>[12x]ETLVRPKPLLLKLLKSVGAQKDTYTMKEVLFYLGQYIMTKRLYDEKQQHIVYCSNDLLGDLFGVPSFSVKEHRKIYTMIYRNLVV;>[12x]XTSFAEYWKLLSCX

Here we report a novel peptide stapling strategy based on the dithiocarbamate chemistry linking the side chains of residues Lys(i) and Cys(i + 4) of unprotected peptides and apply it to a series of dodecameric peptide antagonists of the p53-inhibitory oncogenic proteins MDM2 and MDMX. In this proof-of-concept study, we firstly used PMI – a potent dodecameric peptide antagonist of MDM2 and MDMX that, despite its high affinity for both proteins, fails to activate p53 and kill p53+/+ tumor cells due presumably to its inability to traverse the cell membrane and susceptibility to proteolytic degradation. Previous structural and functional studies of PMI (TSFAEYWNLLSP) identified Phe3, Trp7 and Leu10 as the most critical residues for MDM2/MDMX binding. Crystallographic studies of peptide–MDM2/MDMX complexes structurally validated the chemoselectivity of the dithiocarbamate staple bridging Lys and Cys at (i, i + 4) positions.

Whereas all 12 residues could be built into each PMI(8,12)-a peptide complexed with MDM2, PMI(4,8)-a was fully defined in only 3 copies of the MDMX complex with no density observed for Ser11 and/or Pro12. Alignment analysis of the PMI(8,12)-a conformation also indicated noticeable variability among the 12 copies of peptide, as evidenced by the root-mean-square deviation (RMSD) between the main-chain atoms in the range of 0.48–1.35 Å (Table S3†). In both complexes, however, the crystallographic density for all atoms of the crosslink formed between Lys(i) and Cys(i + 4) unambiguously defined the geometry of the DTC staple. The DTC staple rigidified, at positions (8,12), the C-terminus of PMI in a helical conformation and extended, at positions (4,8), the C-terminal helix of PMI from Leu9 to Ser11. The rigidity of PMI(8,12)-a or PMI(4,8)-a increased to such an extent that the local buried surface area (BSA) slightly decreased as compared with the BSA contributed by PMI to its interface with MDM2/MDMX (Fig. S8†). We deduced the DTC structure of the predominant epimer from the crystal structures of PMI(4,8)-a and PMI(8,12)-a in respective complex with MDMX and MDM2, where Cys8 or Cys12 remained as an l-amino acid residue as shown in the electron density maps. We used HPLC and ESI-MS to evaluate the proteolytic stability of PMI(8,12)-a versus PMI-0 at 100 μM in cell culture medium in the presence of 25 μg ml–1 cathepsin G – an intracellular protease with dual specificities for both basic and bulky hydrophobic residues. As shown in Fig. S9,† while PMI-0 was fully degraded by the enzyme within 30 min of co-incubation at room temperature, the DTC-stapled peptide was substantially more stable with a half-life of ∼8 h under identical conditions.> MSNEVEQKKNIKTINDLPGISQTVINKLIEAGYSSLETLAVASPQDLSVAAGIPLSTAQKIIKEARDALDIRFKTALEVKKERMNVKKISTGSQALDGLLAGGIETRTMTEFFGEFGSGKTQLCHQLSVNVQLPPEKGGLSGKAVYIDTEGTFRWERIENMAKALGLDIDNVMNNIYYIRAINTDHQIAIVDDLQELVSKDPSIKLIVVDSVTSHFRAEYPGRENLAVRQQKLNKHLHQLTRLAEVYDIAVIITNQVMARPDMFYGDPTVAVGGHTLYHVPGIRIQLKKSRGNRR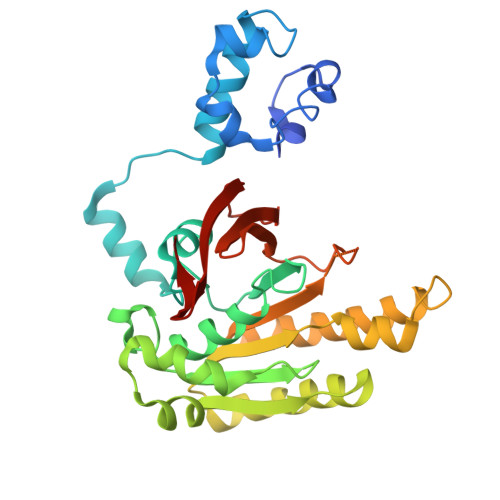IARVVDAPHLPEGEVVFALTEEGIRDAEE> MKHLSDELLIESYFKAKELNLSPEFIELIEKEIQ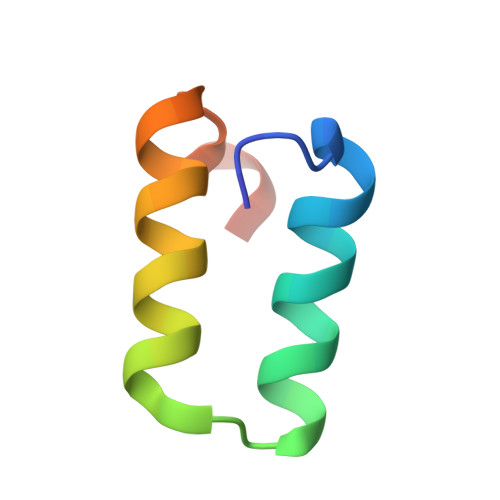RRSLTHKIKLSS>GAGAGAGAGAGMGQPTTTSLFMRDVMFHRMTGTSQAVNDVATLSGERREIIRRALNKKILVPNILELMPAWPSEFQPNIDEVNVEIDEWLKTVNVAKEKKLKHRARGNYTLLAGIYYPHCRKEKMLALSQFLYWIFFWDDEIDTGGELTEDREGTILCCAETNKCINDCLGPEPNYTPPPGSRGTVEMLYPILRDLRAGLSPVSTMRLKQELHDYVNGVKNQQKVRQEDHLPNPWDHFQMRVDDVGVIPSITQNEYAMDFTLPDWIR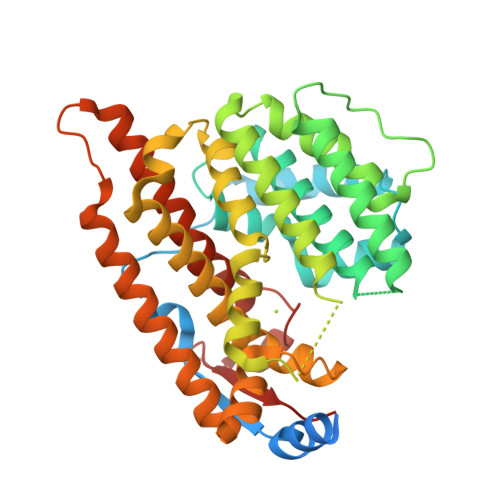RHEAMEEIVLQCTKLTILLNEILSLQKEFRVSQLENLCLLFMNTYDMSIEQSIHKVLGLLKDHYKICIEAEARLPWSTTDEKLNNNIREYIRGCQRLATGTACWSYNCERYFKLSQLNDQQELLLDLSRT[2x]>[2x]GSGSMKDYDELLKYYELHETIGTGGFAKVKLACHILTGEMVAIKIMDKNTLGSDLPRIKTEIEALKNLRHQHICQLYHVLETANKIFMVLEYCPGGELFDYIISQDRLSEEETRVVFRQIVSAVAYVHSQGYAHRDLKPENLLFDEYHKLKLIDFGLCAKPKGNKDYHLQTCCGSLAYAAPELIQGKSYLGSEADVWSMGILLYVLMCGFLPFDDDNVMALYKKIMRGK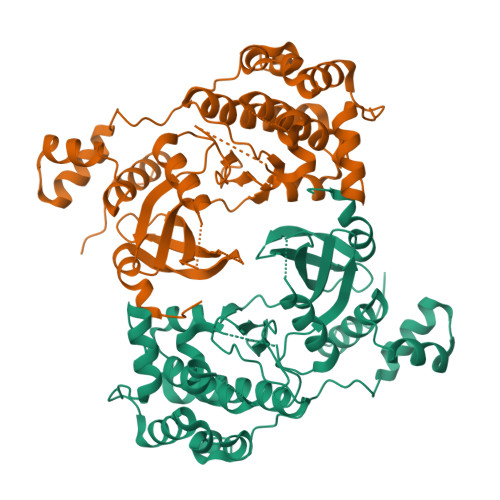YDVPKWLSPSSILLLQQMLQVDPKKRISMKNLLNHPWIMQDYNYPVEWQSKNPFIHLDDDCVTELSVHHRNNRQTMEDLISLWQYDHLTATYLLLLAKKARGKPVRLRLSSFSCG> MKKRGKGVGSMWYGIGNTGLPNPAAAFVEIHGDGSANVMFGAADIGQGSGTAMAQIAAEELGLDYEKIHVTWGDTMVTPDGGATSASRQTLITGNAVILACRQAKETLAKTAAEKLDCAPEELS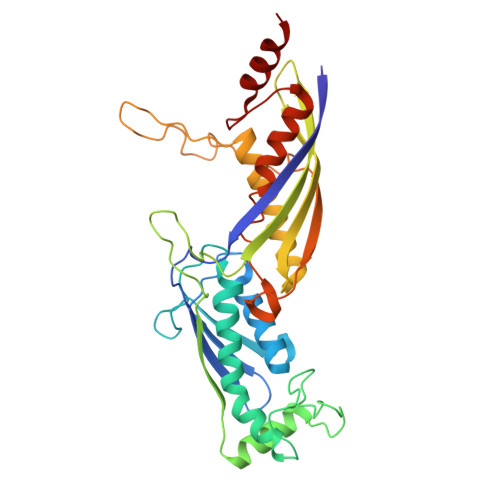FRDNTVFITADPERSMTYGELMAAMKAAGRMAVGAGSYNPNTTGLAPENMSGIPFEVYSYATTIAEVEVDTETGEVDVLKVVSAHDVGTPINRSMVEGQIEGGVTMGQGFVLMEEIEVNTKNGAIKNPSMSKYIIPSNRDVPEIHSILVESEGGPGPFGAKGVGEPALIPMIPAVVAAIEDALGTRFTHTPIMPKDIVAAVKAQEK> TQFEERHLKFLQQLGKGNFGSVEMCRYDPLQDNTGEVVAVKKLQHSTEEHLRDFEREIEILKSLQHDNIVKYKGVCYSAGRRNLKLIMEYLPYGSLRDYLQKHKERIDHIKLLQYTSQICKGMEYLGTKRYIHRDLATRNILVENENRVKIGDFGLTKVLPQDKEYYKVKEPGE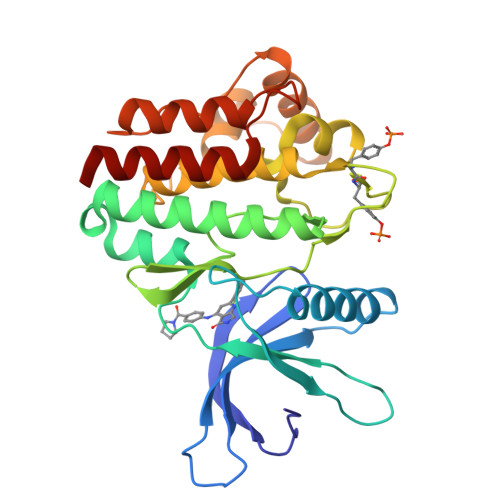SPIFWYAPESLTESKFSVASDVWSFGVVLYELFTYIEKSKSPPAEFMRMIGNDKQGQMIVFHLIELLKNNGRLPRPDGCPDEIYMIMTECWNNNVNQRPSFRDLALRVDQIRDNMAG>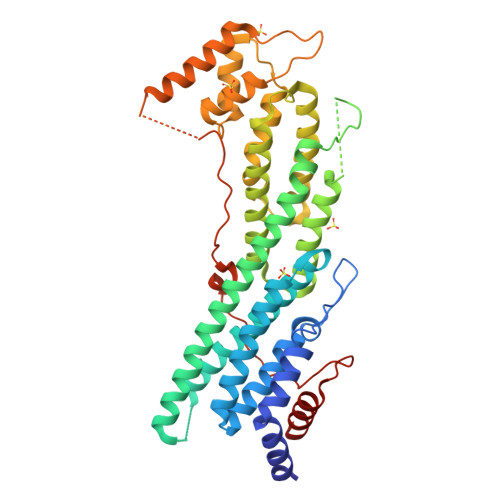 GPGSNATQINEELYRLLEDTEILNQEITEGLLKGFEVPDAGVAIQLSKRDVVYPARILIIVLSEMWRFGLTKQSESFLAQVLTTIQKVVTQLKGNDLIPSGVFWLANVRELYSFVVFALNSILTEETFKNGMTDEEYKEYVSLVTELKDDFEALSYNIYNIWLKKLQKQLQKKAINAVVISESLPGFSAGETSGANTEEYTMDDILTFFNSIYWCMKSFHIENEVFHAVVTTLLNYVDAICFNELIMKRNFLSWKRGLQLNYNVTRLEEWCKTHGLTDGTECLQHLIQTAKLLQVRKYTIEDIDILRGICYSLTPAQLQKLISQYQVADYESPIPQEILRYVADIVKKEAALSSSGNDSKGHEHSSSIFITPETGPFTDPFSLIKTRKFDQVEAYIPAWLSLPSTKRIVDLVAQQVVQDGH> MAVRASEISRVYEAYPEKKATLYFLVLGFLALIVGSLFGPFQALNYGNVDAYPLLKRLLPFVQSYYQGLTLHGVLNAIVFTQLFAQAIMVYLPARELNMRPNMGLMWLSWWMAFIGLVVAALPLLANEATVLYTFYPPLKGHWAFYLGASVFVLSTWVSIYIVLDLWRRWKAANPGKVTPLVTYMAVVFWLMWFLASLGLVLEAVLFLLPWSFGLVEGVDPLV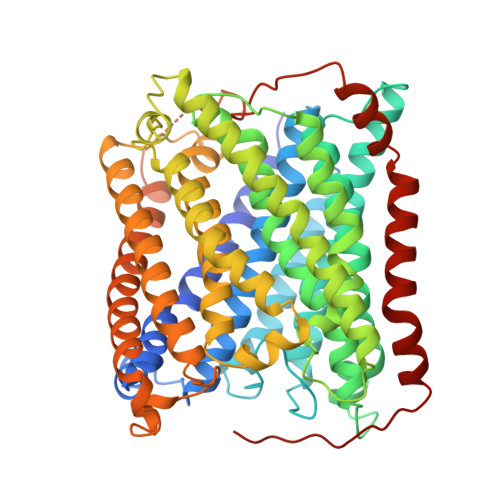ARTLFWWTGHPIVYFWLLPAYAIIYTILPKQAGGKLVSDPMARLAFLLFLLLSTPVGFHHQFADPGIDPTWKMIHSVLTLFVAVPSLMTAFTVAASLEFAGRLRGGRGLFGWIRALPWDNPAFVAPVLGLLGFIPGGAGGIVNASFTLDYVVHNTAWVPGHFHLQVASLVTLTAMGSLYWLLPNLTGKPISDAQRRLGLAVVWLWFLGMMIMAVGLHWAGLLNVPRRAYIAQVPDAYPHAAVPMVFNVLAGIVLLVALLLFIYGLFSVLLSRERKPELAEAPLPFAEVISGPEDRRLVLAMDRIGFWFAVAAILVVLAYGPTLVQLFGHLNPVPGWRLW In bacteria, RuvA, RuvB, and RuvC are involved in processing the HJ. RuvA was shown to assemble into a tetramer for recognizing the HJ core and recruits RuvB. As a motor protein, RuvB can bind the dsDNA part of the HJ and promote the movement of HJ, known as branch migration. RuvB belongs to the AAA+ (ATPase associated with various cellular activities) family, which includes many members involved in numerous physiological processes.

We also incubated RuvB with DNA substrates and 2 mM ATPγS to assemble the RuvB-DNA complex, which was further purified by gel filtration. Data processing in cryoSPARC resulted in two maps with overall resolutions of 2.97 Å and 3.20 Å. These high-resolution maps allowed us to build atomic models of the RuvB-DNA complexes, denoted as RuvB hexamer and RuvB dodecamer models, respectively. The RuvB dodecamer is formed by two RuvB hexamers in a head-to-head manner with approximate dimensions of 158 Å × 127 Å × 127 Å. The RuvB hexamer model resembles RuvB hexamers from the dodecamer with minor differences. Notably, a feature β-hairpin in the NTD of RuvB is invisible in most protomers of RuvB hexamer but is well-defined in all the protomers of RuvB dodecamer. In the RuvB dodecamer, we observed interactions mediated by the feature β-hairpins of RuvB, whereas this feature β-hairpin interacts with the C-terminal domain of RuvA in S. thermophilus RuvB. These interactions, which are absent in our T. thermophilus RuvB hexamer, may stabilize the conformations of the feature β-hairpin in our RuvB dodecamer and in S. thermophilus RuvB. Moreover, the overlaid structures of our RuvB dodecamer and S. thermophilus RuvB showed obvious conformational changes with respect to the feature β-hairpins of equivalent protomers of RuvB. Together, these structural comparisons suggest that the feature β-hairpin of RuvB is conformationally flexible, which may be critical for its unique interaction mode with RuvA in the Holliday junction complex (See section on asymmetric interactions with RuvA). As such, the RuvB dodecamer we obtained is not biologically relevant.

>[12x]MEDLALRPKTLDEYIGQERLKQKLRVYLEAAKARKEPLEHLLLFGPPGLGKTTLAHVIAHELGVNLRVTSGPAIEKPGDLAAILANSLEEGDILFIDEIHRLSRQAEEHLYPAMEDFVMDIVIGQGPAARTIRLELPRFTLIGATTRPGLITAPLLSRFGIVEHLEYYTPEELAQGVMRDARLLGVRITEEAALEIGRRSRGTMRVAKRLFRRVRDFAQVAGEEVITRERALEALAALGLDELGLEKRDREILEVLILRFGGGPVGLATLATALSEDPGTLEEVHEPYLIRQGLLKRTPRGRVATELAYRHLGYPPPVGPLLEP> GAGSDAGQVYRGFIAVMKENFGFIETLSHDEEVFFHFSNYMGNPNWLELGQEVEYTLARNGNTSVSGNCLPAENVRML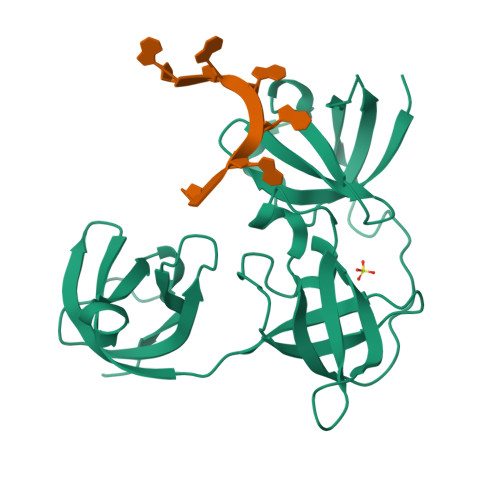PKNSIPQPAVLETTHNGVVARPLRCINPDQQEYAGLIEILDELRTTVISQHEFGITSLVNKRDLLQKGDLVSFRIDESGRAACVNAVRQKKRATVDSIKGQFGFLNFEVEDGKKLFFHMSEVQGNTVALHPGDTVEFSVVTNQRNGKSSACNVLKIND>ETQPQMFFGVLDREELEYFKQAESTLQLDAFEAPEEKFQFVTSIIEEAKGKELKLVTSQITSKLMERVILECDETQLKDIFQSFNGVFFGLSCHKYASHVLETLFVRSAALVERELLTPSFDNNEKEGPYVTMENMFLFMLNELKPHLKTMMNHQYASHVLRLLILILSSKTLPNSTKANSTLRSKKSKIARKMIDIKDNDDFNKVYQTPESFKSELRDIITTLYKGFTNGAESRSDISQSTITKFREYSVDKVASPVIQLIIQVEGIFDRDRSFWRLVFNTADEKDPKEESFLEYLLSDPVGSHFLENVIGSARLKYVERLYRLYMKDRIVKLAKRDTTGAFVVRALLEHLKEKDVKQILDAVVPELSMLLNSNMDFGTAIINTSNKQGGYLRDDVIAQLIQKYYPEKSDAKNILESCLLLSASTLGNTRDDWPTAEERRRSVFLEQLIDYDDKFLNITIDSMLALPEERLIQMCYHGVFSHVVEHVLQTTRVDIIKRKMLLNILSKESVNLACNVYGSHIMDKLWEFTAKLTLYKERIARALVLETEKVKNSIYGRQVWKNWKLELYVRKMWDWKKLIKEQEFEIFPNSKPLQPKPEK[2x]

Nop9, a nucleolar protein conserved in humans, plants and yeast, is essential for 18S rRNA maturation. Nop9 represents one of three distinct subfamilies of Pumilio/fem-3 mRNA-binding factor (PUF) proteins, along with the classical PUF and the Puf-A/Puf6 subfamilies. Consistent with a role in processing 20S pre-rRNA to mature 18S rRNA, we find that Nop9 binds to the fragment of internal transcribed spacer 1 (ITS1) present in the 20S pre-rRNA. Moreover, the presence of Nop9 reduces the cleavage efficiency of Nob1 in vitro. Together, our results suggest that Nop9's essential role in SSU ribosome biogenesis is to prevent premature cleavage of the 20S pre-rRNA by Nob1 in the nucleolus.

We determined a 2.1-Å-resolution crystal structure of yeast Nop9 that revealed a new PUM repeat fold with 11 PUM repeats (R1 to R11) arranged in a C-like shape. The repeats form a twisted, incomplete ring with an ∼80-Å outer diameter, an ∼35 Å inner diameter and 30–40 Å thickness. Most of the individual PUM repeats are similar to classical PUM repeats with three α helices, but with variability in the length of helices and interhelix loops. The repeats form a curved overall structure, and twisting relative to imaginary repeat-to-repeat axes is focused at repeats R4 and R7. Extended loops before and after repeat R4 and a long loop between repeats R7 and R8 each correspond to ∼25° twists. Repeat R11 diverges in structure from a classical PUM repeat with two α helices at the C-terminal end that cap the structure. Two long loops between helices α2 and α3 in repeats R2 (residues 164–174) and R3 (residues 220–250) are disordered in the crystal structure. The most-conserved residues across Nop9 family proteins are found on the inner concave surface at the positions that typically recognize RNA bases in classical PUF proteins. The most common motif in Nop9, SϕxxE/D (where ϕ is a stacking side chain and x is a hydrophobic side chain), specifies a G base in classical PUF proteins such as PUM1. This motif is found in repeats R1, R2, R5 and R8-R10 of Nop9.> EKSVVFKAEGEHFTDQKGNTIVGSGSGGTTKYFRIPAMCTTSKGTIVVFADARHNTASDQSFIDTAAARSTDGGKTWNKKIAIYNDRVNSKLSRVMDPTCIVANIQGRETILVMVGKWNNNDKTWGAYRDKAPDTDWDLVLYKSTDDGVTFSKVETNIHDIVTKNGTISAMLGGVGSGLQLNDGKLVFPVQMVRTKNIT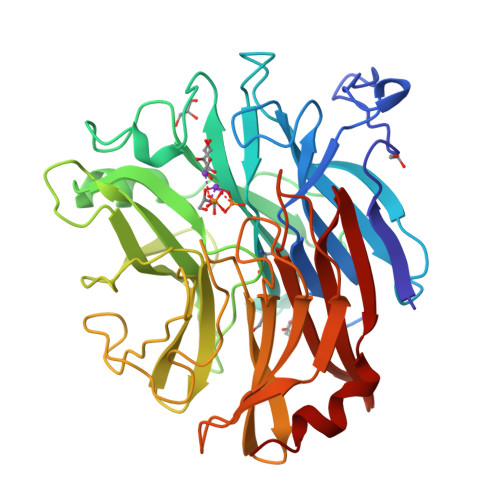TVLNTSFIYSTDGITWSLPSGYCEGFGSENNIIEFNASLVNNIRNSGLRRSFETKDFGKTWTEFPPMDKKVDNRNHGVQGSTITIPSGNKLVAAHSSAQNKNNDYTRSDISLYAHNLYSGEVKLIDDFYPKVGNASGAGYSCLSYRKNVDKETLYVVYEANGSIEFQDLSRHLPVIKSYN> MDLERLAQRLEGLGG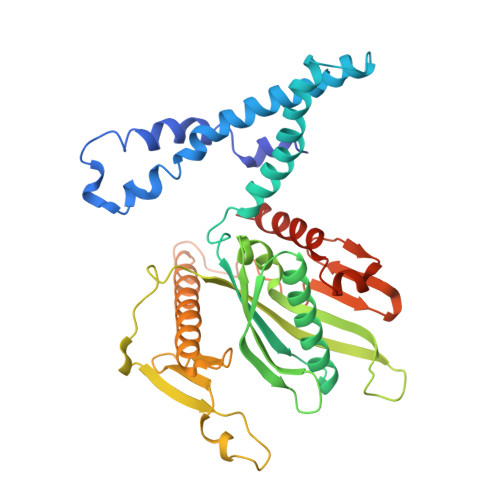IFDIPQKETRLKELERRLEDPSLWNDPEAARKVSQEAARLRRTVDTFRSLESDLQGLLELMEELPAEEREALKPELEEAAKKLDELYHQTLLNFPHAEKNAILTIQPGAGGTEACDWAEMLLRMYTRFAERQGFQVEVVDLTPGPEAGIDYAQILVKGENAYGLLSPEAGVHRLVRPSPFDASGRRHTSFAGVEVIPEVDEEVEVVLKPEELRIDVMRASGPGGQGVNTTDSAVRVVHLPTGITVTCQTTRSQIKNKELALKILKARLYELERKKREEELKALRGEVRPIEWGSQIRSYVLDKNYVKDHRTGLMRHDPENVLDGDLMDLIWAGLEWKAGRRQGTEEVEAE>[2x]GSHMKVMFIPSRAVPFNPDRVQGGLEAVHLNVLKYLVSIGADIDYIGFDNDTFGDWKVTHHPV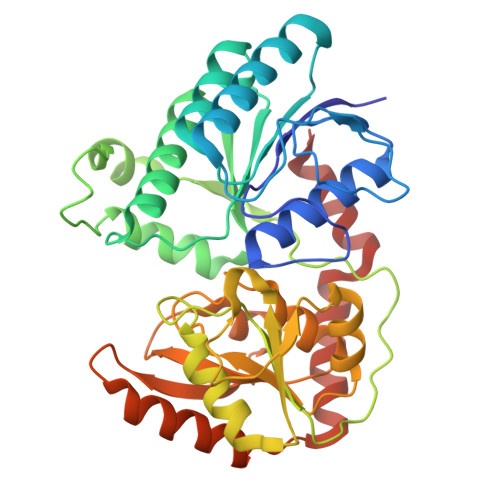GHLTKFSLGMSYTMARKIVELAGIHEYDFVVTMEPTKLTVQAIKDAGLSKVHKNFMATPFEPVSRGIVQIWDQTIQIHKNGGKSYAPTKAFREFERKYCHMTSALTDKIDYDYWRANPLFEAEDYPVICLNEKPEVLPATDLIISAQRYDTKMRRTDVALEAIKALGENGVGYCPSKWAPPAKYPVIIDAPHSEIMERLKTAKALINTCPDTGTVENSSIEAISKGVPVIQLVFKDYPHATFEYDPDTVRVEIDFSTPKKEVVALYTKAVLEFTDTYEARVKRAEAVWKKYNRDAVVAMWDKIFTA THIOUREA | C H4 N2 S | 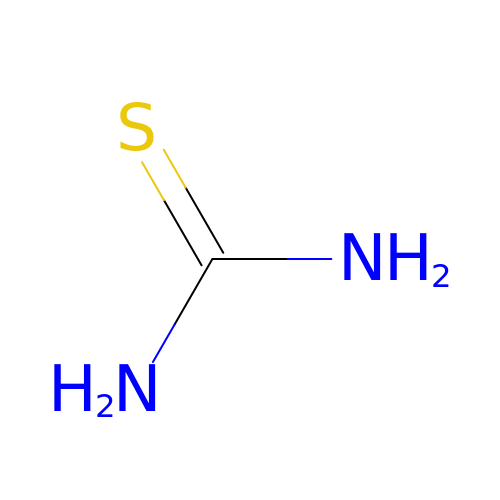UMGDCJDMYOKAJW-UHFFFAOYSA-N>MSVKAHESVMDWVTEELRSGRLKIGDHLPSERALSETLGVSRSSLREALRVLEALGTISTATGSGPRSGTIITAAPGQALSLSVTLQLVTNQVGHHDIYETRQLLEGWAALHSSAERGDWDVAEALLEKMDDPSLPLEDFLRFDAEFHVVISKGAE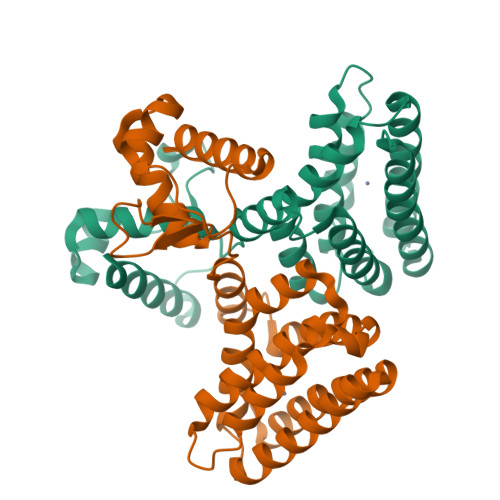NPLISTLMEALRLSVADHTVARARALPDWRATSARLQKEHRAILAALRAGESTVAATLIKEHIEGYYEETAAAEALEHHHHHH[2x]> WMDF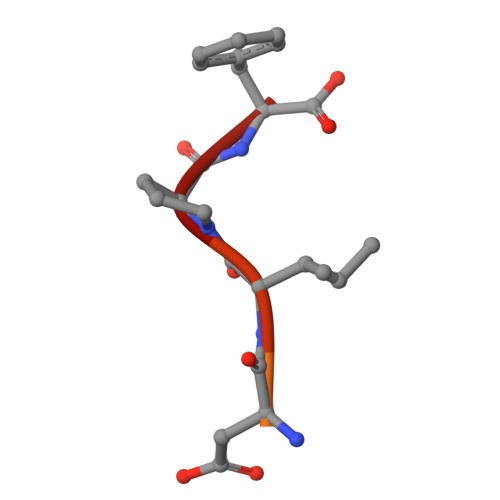DDDIPF A major factor that limits the expansion of shrimp cultures is, however, infectious diseases from viruses, such as P. vannamei nodavirus (PvNV) and M. rosenbergii nodavirus (MrNV), which have inflicted heavy economic losses. The Nodaviridae genome comprises two single-stranded positive-sense RNA that encode the capsid protein for viral capsid assembly, the RNA polymerase for RNA replication, and the B2 protein for host RNA interference suppressor. While the shell domains (S-domains) of PvNV and MrNV contain conserved sequences of 62% identity, the protrusion domains (P-domains) and N-arms show low sequence identities of only 17% and 43%, respectively. In this work, we have determined the cryo-EM structures of T = 3 and T = 1 PvNV-LPs at atomic resolution, the crystal structures of the P-domains of PvNV and MrNV (PvNVPd and MrNVPd), and the crystal structure of the S-domain of PvNV (ΔN-ARM-PvNVSd) in the T = 1 subviral particle (SVP).

As for the MrNvPd, three crystal forms (P3221, C2221, and P4332) were determined. The structure of MrNVPd (P3221) was determined by Se-SAD, independently from PvNVPd, and all structures were refined to 1.39–2.3 Å resolutions. First, the high-resolution crystal structure (P3221) allows us to locate clearly the metal ions. The 311ExD313 motif on turn β4/β5 interacts with one Zn2+ ion through direct electrostatic interactions. Glu270 on turn β1/β2 and Asp355 on turn β7/β8 also coordinate with Zn2+ ions. The distances between the Zn2+ ions and the side chains of Glu270, Glu341 and Asp355 from three separate asymmetric units are ~2.4 Å, which is in a reasonable range for a Zn2+/ligand coordination. In addition, these three key residues are involved in another Zn2+-binding site located at the intermolecular interface of two MrNVPd dimers. Similar to PvNVPd, the symmetry of MrNVPd dimers (P3221) also generates a dimer–dimer conformation, but with additional metal ions coordinated in the dimer–dimer interface and with a slightly altered bending angle of ~120°. Three key residues Glu270, Glu341, and Asp355 reveal a negatively charged interface and work together with three Zn2+ ions through hydrogen bonds connecting three turns β1/β2, β6/β7, and β7/β8, respectively. Examination of the intermolecular MrNVPd dimer–dimer interaction reveals that Glu270, Glu341, and Asp355 donate major hydrogen bonds to stabilize this conformation (with the exception of the 311ExD313 motif), suggesting that the negatively charged Asp313 on the MrNVPd monomer might exist as a potential metal-binding site without participating in the MrNVPd dimer–dimer structure.

> PTPVEVSQLTYNADTIGNWVPPTELKQTYTQDITGLKPNSKFIIVPYMDRVSSEVLQKCTITCNEVDAVGSISYFDTSAIKCDGYISFQANSIGEATFTLVTDYQGAVDPKPYQYRIIRAIVGNN>SERFPNDVDPIETRDWLQAIESVIREEGVERAQYLIDQLLAEARKGGVNVAAGTGISNYINTIPVEEQPEYPGNLELERRIRSAIRWNAIMTVLRASKKDLELGGHMASFQSSATIYDVCFNHFFRARNEQDGGDLVYFQGHISPGVYARAFLEGRLTQEQLDNFRQEVHGNGLSSYPHPKLMPEFWQFPTVSMGLGPIGAIYQAKFLKYLEHRGLKDTSKQTVYAFLGDGEMDEPESKGAITIATREKLDNLVFVINCNLQ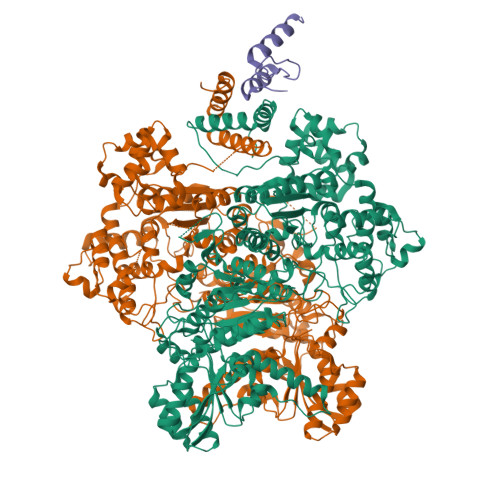RLDGPVTGNGKIINELEGIFEGAGWNVIKVMWGSRWDELLRKDTSGKLIQLMNETVDGDYQTFKSKDGAYVREHFFGKYPETAALVADWTDEQIWALNRGGHDPKKIYAAFKKAQETKGKATVILAHTIKGYGMGDAAEGKNIAHQVKKMNMDGVRHIRDRFNVPVSDADIEKLPYITFPEGSEEHTYLHAQRQKLHGYLPSRQPNFTEKLELPSLQDFGALLEEQSKEISTTIAFVRALNVMLKNKSIKDRLVPIIADEARTFGMEGLFRQIGIYSPNGQQYTPQDREQVAYYKEDEKGQILQEGINELGAGCSWLAAATSYSTNNLPMIPFYIYYSMFGFQRIGDLCWAAGDQQARGFLIGGTSGRTTLNGEGLQHEDGHSHIQSLTIPNCISYDPAYAYEVAVIMHDGLERMYGEKQENVYYYITTLNENYHMPAMPEGAEEGIRKGIYKLETIEGSKGKVQLLGSGSILRHVREAAEILAKDYGVGSDVYSVTSFTELARDGQDCERWNMLHPLETPRVPYIAQVMNDAPAVASTDYMKLFAEQVRTYVPADDYRVLGTDGFGRSDSRENLRHHFEVDASYVVVAALGELAKRGEIDKKVVADAIAKFNIDADKVNPRLA[4x];>[2x]VHATPLIRRLAREFGVNLAKVKGTGRKGRILREDVQAYVKEAIKRA> DYKDDDDAMANSASPEQNQNHCSAINNSIPLMQGNLPTLTLSGKIRVTVTFFLFLLSATFNASFLLKLQKWTQKKEKGKKLSRMKLLLKHLTLANLLETLIVMPLDGMWNITVQWYAGELLCKVLSYLKLFSMYAKAFMMVVISLDRSLAITRPLALKSNSKVGQSMVGLAWILSSVFAGPQLYIFRMIHLADSSGQTKVFSQCVTHCSFSQWWHQAFYNFFTFSCLFIIPLFIMLICNAKIIFTLTRVLGIDCSFWNESYLTGSRDERKKSLLSKFGMDEGVTFMFIGRFDRGQKGVDVLLKAIEILSSKKEFQEMRFIIIGKGDPELEGWARSLEEKHGNVKVITEMLSREFVRELYGSVDFVIIPSYFEPFGLVALEAMCLGAIPIASAVGGLRDIITNETGILVKAGDPGELANAILKALELSRSDLSKFRENCKKRAMSFSNIPRARLKTLKMTVAFATSFTVCWTPYYVLGIWYWFDPEMLNRLSDPVNHFFFLFAFLNPCFDPLIYGYFSLHHHHHHHHHH

The central regulator of the HPG axis is gonadotrophin-releasing hormone (GnRH), a decapeptide neurohormone produced by mammalian hypothalamus neurons. The GnRH peptide can activate the GnRH receptor through the heterotrimeric Gq protein pathway. There are two isoforms of the GnRH peptide in humans, GnRH-I and GnRH-II, and their effects are exerted by activation of the classical GnRH1 receptor (GnRH1R), which belongs to the rhodopsin G protein-coupled receptor (GPCR) family. GnRH1R is expressed primarily on pituitary gonadotrope cells but also on lymphocytes and breast, ovary, and prostate cells, and has emerged as a promising therapeutic target for the treatment of conditions including infertility, uterine fibroids, endometriosis, and prostate cancer.

In this study, we report the crystal structure of human GnRH1R in complex with the antagonist drug elagolix. For lipidic cubic phase (LCP) crystallization, an initial GnRH1R construct was generated by replacing the third intracellular loop (ICL3; amino acids [aa] 243–256) with the thermostable Pyrococcus abysi glycogen synthase (PGS) domain22. To further improve the homogeneity of the receptor, the point mutation P1283.39K (Ballesteros–Weinstein numbering used in superscript) was incorporated into the engineered construct and the position 3.39 mutants were previously shown to make receptors stable in an inactive state, and were also reported in other recently elucidated GPCR structures. Finally, GnRH1R (P1283.39K)-PGS was crystallized using the LCP method in the presence of elagolix and the structure was successfully determined at 2.8 Å resolution. The overall architecture of full-length GnRH1R consists of seven canonical transmembrane (TM) helices but lacks a cytoplasmic C-terminal helix (helix 8). In summary, the GnRH1R crystallized in complex with the antagonist drug elagolix represents an inactive conformation with respect to G protein coupling. In contrast to the previously reported structures of β-branch class A GPCRs, one interesting feature of GnRH1R on the extracellular side is that the N-terminal region (aa 18–33) before TM1 is well folded and inserted into the orthosteric binding cavity with clear electron density in the structure. The overall pocket in GnRH1R is defined by the N terminus, TM2, TM3, TM5, TM6, and TM7, forming a highly hydrophobic binding site. The pyrimidine ring, as the core of the ligand elagolix, sits above the aromatic side chain of Y2836.51 and forms a hydrophobic π–π interaction with each other. However, the oxygen atom at position 4 is engaged in binding with the side chains of residues K1213.32 and D982.61, forming only a polar interaction network in the elagolix binding site.>[3x]MGSSHHHHHHENLYFQGSMEQAIINDEREYLRHFWHPVCTVTELEKAHPSSLGPLAVKLLNEQLVVAKLGDEYVAMRDRCAHRSAKLSLGTVSG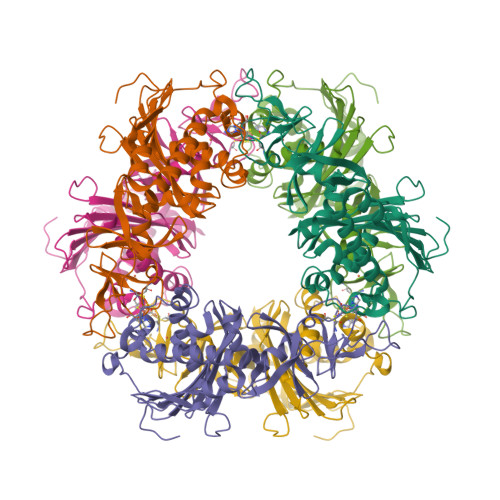NRLQCPYHGWQYDTHGACQLVPACPNSPIPNKAKVDRFDCEERYGLIWIRLDSSFDCTEIPYFSAANDPRLRIVIQEPYWWDATAERRWENFTDFSHFAFIHPGTLFDPNNAEPPIVPMDRFNGQFRFVYDTPEDMAVPNQAPIGSFSYTCSMPFAINLEVSKYSSSSLHVLFNVSCPVDSHTTKNFLIFAREQSDDSDYLHIAFNDLVFAEDKPVIESQWPKDAPADEVSVVADKVSIQYRKWLRELKEAHKEGSQAFRSALLDPVIESDRSYI> MKKFASLILTSVFLFSSTQFVHASSTDVQERLRDLAREDEAGTFNEAWNTNFKPSDEQQFSYSPTEGIVFLTPPKNVIGERRISQYKVNNAWATLEGSPTEASGTPLYAGKNVLDNSKGTMDQELLTPEFNYTYTESTSNTTTHGLKLGVKTTATMKFPIAQGSMEASTEYNFQNSSTDTKTKQVSYKSPSQKIKVPAGKTYRVLAYLNTGSISGEANLYANVGGIAWRVSPGYPNGGGVNIGAVLTKCQQKGWGDFRNFQPSGRDVIVKGQGTFKSNYGTDFILKIEDITDSKLRNNNGSGTVVQEIKVPLIRTEIHHHHAHHH

Mpp75Aa1.1 (formerly known as Cry75Aa1.1), discovered by mining the genome of Brevibacillus laterosporus, provides effective control of WCR larvae when expressed in transgenic maize. Bioinformatic analysis identified that Mpp75Aa1.1 belongs to the aerolysin-like superfamily of bacterial beta-pore forming proteins (β-PFPs) found across all kingdoms of life. More specifically, the Pfam (Protein family) database classification indicates that it is a member of the ETX_MTX2 sub-family of β-PFPs. The Mpp75Aa1.1 is processed at its carboxyl-terminus by WCR midgut proteases, forms an oligomer, and specifically interacts with putative membrane-associated binding partners on the midgut apical microvilli to cause cellular tissue damage resulting in insect death.

The crystal structure of Mpp75Aa1.1 was solved at 1.94 Å resolution using the SAD heavy atom phasing method from a crystal briefly soaked in samarium acetate. The protein crystallized in tetragonal crystal lattice of space group P4322 with one molecule in the asymmetric unit. The Mpp75Aa1.1 structure revealed an overall elongated shape with approximate dimensions of 112 Å x 26 Å x 22 Å with a high prevalence of β-strands. The molecule is composed of three structural domains. Domain I, corresponding to the head region of the molecule, displays a non-contiguous fold encompassing four alpha-helices (α1-α4) and six short β-strands (β1-β3 and β14-β16). Domain II, at the center of Mpp75Aa1.1, is characterized by a set of anti-parallel β-strands running longitudinal across two-thirds of the Mpp75Aa1.1 structure, and a two-stranded anti-parallel β-hairpin (β9 and β10) which amino acid constituents are amphipathic, with alternating hydrophobic and hydrophilic residues. Domain III, localized at the tail-end of Mpp75Aa1.1, contains a carboxyl terminal peptide (CTP), β-strands β18, β19, and β20 (β20 corresponds to an introduced histidine tag). Domains II-III adopts a topology representing the conserved structural core of the aerolysin-like proteins. We observed a more extended C-terminal peptide that encircles parts of domain II of Mpp75Aa1.1 via hydrogen bonded interactions between β17 and β18 as well as β20 and β11 (excluding the his-tag residues), whereas ETX has a C-terminal peptide that folds back on itself, thereby reducing the extent of the interactions with the adjacent domain II β-strands. Furthermore, the Mpp75Aa1.1 structure also revealed that WCR-specificity is likely conferred by three domain I residues in the β14 (W206), β15 (G217) strands as well as in the connecting unstructured loop (Y212), which are located at a different part of domain I.>[2x]GSWEIDPKDLTFLKELGTGQFGVVKYGKWRGQYDVAIKMIKEGSMSEDEFIEEAKVMMNLSHEKLV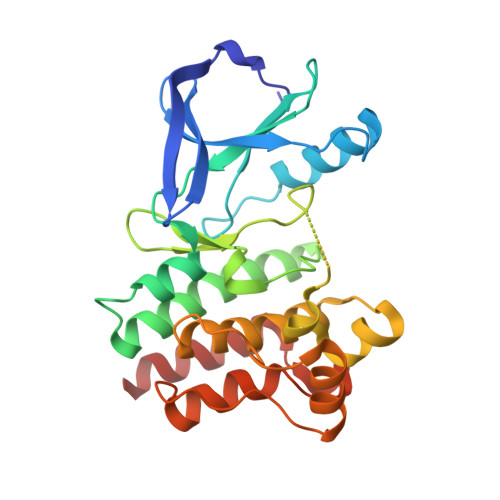QLYGVCTKQRPIFIITEYMANGCLLNYLREMRHRFQTQQLLEMCKDVCEAMEYLESKQFLHRDLAARNCLVNDQGVVKVSDFGLSRYVLDDEYTSSVGSKFPVRWSPPEVLMYSKFSSKSDIWAFGVLMWEIYSLGKMPYERFTNSETAEHIAQGLRLYRPHLASEKVYTIMYSCWHEKADERPTFKILLSNILDVMDEES>[4x]MWSHPAVRKSSSKTIRSRSIWDDAHAMLEKAKAEGISTVWDRAAEQTPACKFCELGTTCRNCIMGPCRIANRKDGKMRLGVCGADADVIVARNFGRFIAGGAAGHSDHGRDLIETLEAVAEGKAPGYTIRDVAKLRRIAAELGVADAATRPAHDVAADLVTICYNDFGSRRNALAFLARAPQVRRDLWQRLGMTPRGVDREIAEMMHRTHMGCDNDHTSLLVHAARTALADGWGGSMIGTELSDILFGTPRPRQSTVNLGVLRKDAVNILVHGHNPVVSEMILAATREPAVRQAAQDAGAADINVAGLCCTGNELLMRQGIPMAGNHLMTELAIVTGAADAIVADYQCIMPSLVQIAACYHTRFVTTSPKGRFTGATHVEVHPHNA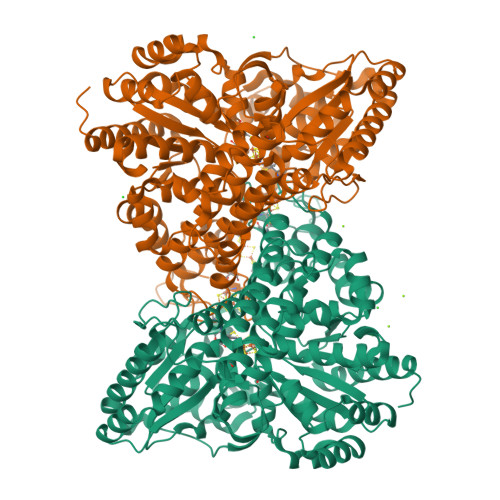QERCREIVMLAIDAYTRRDPARVDIPSQPVSIMSGFSNEAILEALGGTPKPLIDAVVAGQIRGFVGIVGCNNPKIRQDSANVTLTRELIRRDIMVLATGCVTTAAGKAGLLVPEAASKAGEGLAAVCRSLGVPPVLHMGSCVDNSRILQLCALLATTLGVDISDLPVGASSPEWYSEKAAAIAMYAVASGIPTHLGLPPNILGSENVTAMALHGLQDVVGAAFMVEPDPVKAADMLEAHIVARRARLGLTS> LDFDILTNDGTHRNMKLLIDLKNIFSRQLPKMPKEYIVKLVFDRHHESMVILKNKQKVIGGICFRQYKPQRFAEVAFLAVTANEQVRGYGTRLMNKFKDHMQKQNIEY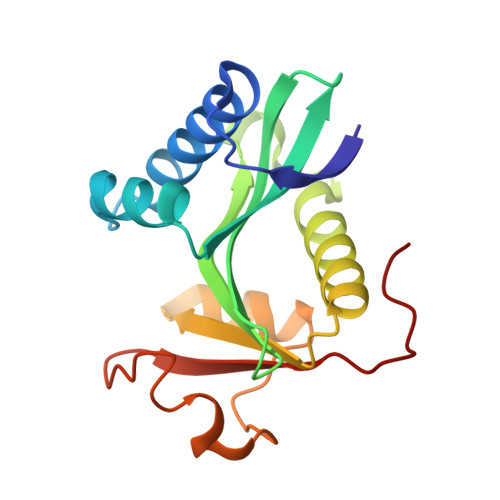LLTYADNFAIGYFKKQGFTKEHRMPQEKWKGYIKDYDGGTLMECYIHPYVDYGR The neuraminidase inhibitors (NAIs) oseltamivir and zanamivir are the antiviral agents available in France to treat influenza A or B virus infections. The NA active site includes catalytic residues (R118, D151, R152, R224, E276, R292, R371, and Y406; N2 numbering) that interact directly with the sialic acid substrate and framework residues (E119, R156, W178, S179, D/N198, I222, E227, H274, E277, N294, and E425; N2 numbering) that stabilize the active site. NAs are divided into 3 phylogenic groups: influenza B viruses, group 1 (N1, N4, N5, and N8), and group 2 (N2, N3, N6, N7, and N9) from influenza A viruses. I221 (B NA numbering), I222 (N2 numbering), and I223 (N1 numbering) amino acids are highly conserved framework residues in NAs of influenza viruses.

We used X-ray crystallography to understand the structural basis of resistance to oseltamivir conferred by NA carrying the I221L substitution. The structure of the NA-I221L-oseltamivir complex showed that the L side chain protrudes into the hydrophobic pocket of the active site that accommodates the pentyloxy substituent of oseltamivir, thus causing a change in the conformation of the inhibitor such that its C81 carbon moves about 2.2 Å from the wild-type NA bound position.

>[2x]MLPSTIQTLTLFLTSGGVLLSLYVSASLSYLLYSDILLKFSPTEITAPTMPLDCANASNVQAVNRSATKGVTLLLPEPEWTYPRLSCPGSTFQKALLISPHRFGETKGNSAPLIIREPFIACGPNECKHFALTHYAAQPGGYYNGTRGDRNKLRHLISVKLGKIPTVENSIFHMAAWSGSACHDGKEWTYIGVDGPDNNALLKVKYGEAYTDTYHSYANKILRTQESACNCIGGNCYLMITDGSASGVSECRFLKIREGRIIKEIFPTGRVKHTEECTCGFASNKTIECACRDNSYTAKRPFVKLNVETDTAEIRLMCTDTYLDTPRPNDGSITGPCESNGDKGSGGIKGGFVHQRMESKIGRWYSRTMSKTERMGMGLYVKYDGDPWADSDALAFSGVMVSMKEPGWYSFGFEIKDKKCDVPCIGIEMVHDGGKETWHSAATAIYCLMGSGQLLWDTVTGVDMAL> NAQVPTEEVSLEVLLSNGQKVLVNVLTSDQTEDVLEAVAAKLDLPDDLIGYFSLFLVREKEDGAFSFVRKLQEFELPYVSVTSLRSQEYKIVLRKSYWDSAYDDDVMENRVGLNLLYAQTVSDIERGWILVTKEQHRQLKSLQEKVSKKEFLRLAQTLRHYGYLRFDACVADFPEKDCPVVVSAGNSELSLQLRLPGQQLREGSFRVTRMRCWRVTSSVPLPSGSTSSPGRGRGEVRLELAFEYLMSKDRLQWVTITSPQAIMMSIC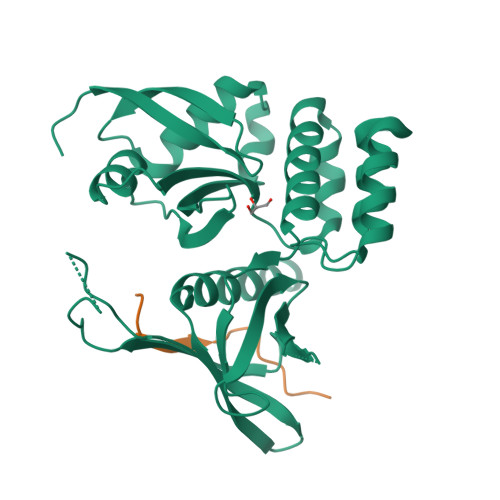LQSMVDELMVKKS;> GASAGSSKRLRKKDDGKCPLNPHSHLGTYGVFTNAAYDPTP> MERNKLARQIIDTCLEMTRLGLNQGTAGNVSVRYQDGMLITPTGIPYEKLTESHIVFIDGNGKHEEGKLPSSEWRFHMAAYQSRPDANAVVHNHAVHCTAVSILNRSIPAIHYMIAAAGGNSIPCAPYATFGTRELSEHVA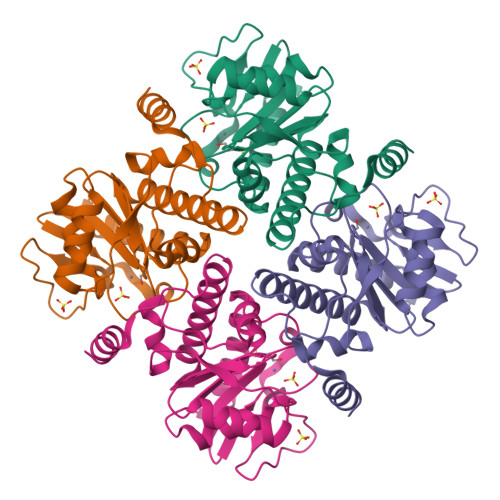LALKNRKATLLQHHGLIACEVNLEKALWLAHEVEVLAQLYLTTLAITDPVPVLSDEEIAVVLEKFKTYGLAIEE7-METHYL-2H-ISOQUINOLIN-1-ONE | C10 H9 N 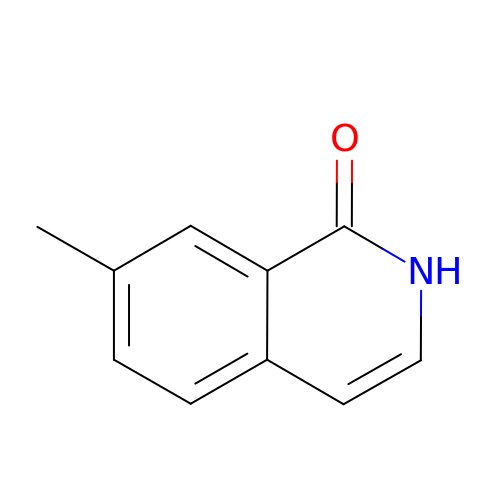O | ZLTCEYHTNOZGIS-UHFFFAOYSA-N>[2x]MPTLLLTGFEPFHTHPDNPSAQAAQELHGLELPGGWGVHS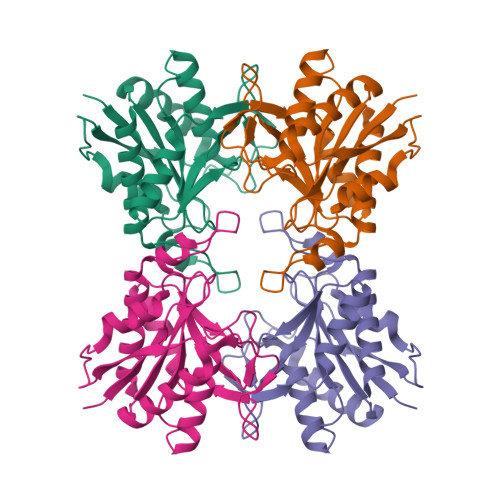ALLPVEPHAAGAALTRLLSEQDPGAVLLTGLAAGRPQVTLERVGVGVMDFQIPDNAGQTYRDQPIEPDAPAAYLATLPLRAILAAWREAEIPGDISNSAGLYVCNFVLYHALHWLREHGRGAVPCGFLHVPANAAVALAVPADRPPLPYLPQSEITRAVRVAAEAITAQSSVLQMGKM>GSAKDPMEKFIKQFSFIALENIFRELPNKITHSFNDINDIKPPKLMYPIFYGSYDWHSSVHSHWLLVKILKDFSHFAPKDEIIKALDSQFSKEKAEGELKYLQNPAHKGFERPYGWGWFLKLTLEINLLAKENDKAEIWAKNLEGIADFFVKEFKEFLPKMDYPIRVGTHFNSSFALYFALEYARFKKDQELEYCIIQSAKKWFLSDKNMQALEPCGDEFLSPVLMEAVLLSAVLHKNDFVKFFKAYLPNLEAKEPATLFTPVSVSDRSDGKIAHLDGLNLSRAWCFKILSNFCDENLKILLRNNATEHFDKAIAHIEDDYLGSHWLGSFALL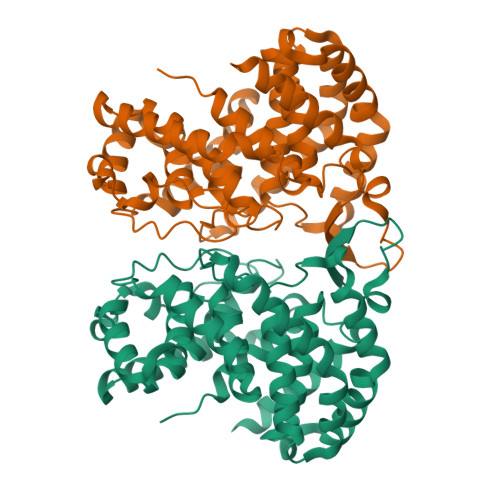ALDVDIL[6x]>MKIVLVLYDAGKHAADEEKLYGCTENKLGIANWLKDQGHELITTSDKEGGNSVLDQHIPDADIIITTPFHPAYITKERIDKAKKLKLVVVAGVGSDHIDLDYINQTGKKISVLEVTGSNVVSVAEHVLMTMLVLVRNFVPAHEQIINHDWEVAAIAKDAYDIEGKTIATIGAGRIGYRVLERLVPFNPKELLYYDYQALPKDAEEKVGARRVENIEELVAQADIVTINAPLHAGTKGLINKELLSKFKKGAWLVNTARGAICVAEDVAAALESGQLRGYGGDVWFPQPAPKDHPWRDMRNKYGAGNAMTPHYSGTTLDAQTRYAEGTKNILE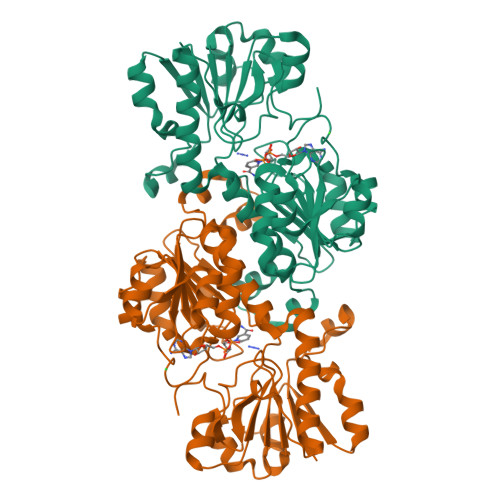SFFTGKFDYRPQDIILLNGEYITKAYGKHDKK[2x]>SNLVLYTLHLSPPCRAVELTAKALGLELEQKTINLLTGDHLKPEFVKLNPQHTIPVLDDNGTIITESHAIMIYLVTKYGKDDSLYPKDPVKQARVNSALHFESGVLFARMRFTFERILFFGKSDIPEDRVEYVQKSYELLEDTLVDDFVAGPTMTIADFSCISTVSSIMGVVPLEQSKHPRIYAWIDRLKQLPYYEEVNGGGGTDLGKFVLAKKEENAKA[4x]

An epsilon-class glutathione-S-transferase in An. gambiae, GSTE2, and its orthologue in the dengue and yellow fever vector Aedes aegypti, have been linked to DDT resistance through elevated gene expression. Recombinant protein expression and in vitro assays also support a role for this enzyme in DDT metabolism. Upon review of the crystal structure that was already resolved for GSTE2 from the susceptible Kisumu strain, it appeared that the alleles differed in codons proximal to the putative DDT-binding site, a hydrophobic pocket adjacent to the glutathione (GSH) binding site. Previously, Wang et al. proposed that a hydrophobic pocket in close proximity to the GSH binding site was the site of DDT binding.

Our study focused upon two residue exchanges, I114T and F120L, which are located in the C-terminal section of helix H4 and, thus, have the potential to influence DDT binding. Position 114 is also situated in close proximity to the predicted DDT binding pocket. In this case, a destabilizing polar hydroxyl group is introduced in a hydrophobic core region of the protein in ZAN/U, with the potential for marked effects on protein conformation. To better uNderstand the effect of this substitution in enzyme activation, we elucidated the structure of ZAN/U:GSH using X-ray crystallography. Interestingly, inspection of electron density maps for all GSTE2 enzymes, calculated using PDB_REDO, reveal a disorder of residues F113 and Y133, which are involved in the mutual packing of two H4 helices across the dimer interface, at a spot that is immediately local to the predicted DDT pocket. This suggests that this region, which constitutes the DDT pocket ‘cap’, has high intrinsic dynamics. Our data suggest that mutations can influence catalysis even when not resulting in detectable structural alterations, most likely by affecting the molecular dynamics of this region. The I114T change was predicted as strongly destabilising at 2.85 kcal/mol, while the F120L was classified as neutral at –0.98 kcal/mol. The importance of mutation I114T most likely arises from the creation of an enzyme with increased catalytic activity through predicted increased conformation dynamics and reduced product affinity, facilitating metabolic turnover.> GIDPFTMAGAEWKSLEECLEKHLPLPDLQEVKRVLYGKELRKLDLPREAFEAASREDFELQGYAFEAAEEQLRRPRIVHVGLVQNRIPLPANAPVAEQVSALHRRIKAIVEVAAMCGVNIICFQEAWTMPFAFCTREKLPWTEFAESAEDGPTTRFCQKLAKNHDMVVVSPILERDSEHGDVLWNTAVVISNSGAVLGKTRKNHIPRVGD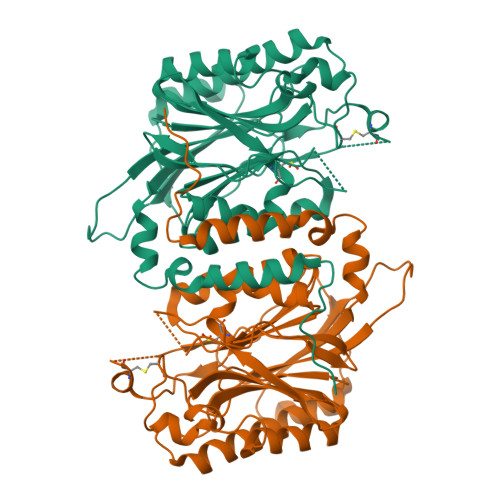FNESTYYMEGNLGHPVFQTQFGRIAVNICYGRHHPLNWLMYSINGAEIIFNPSATIGALSESLWPIEARNAAIANHCFTCAINRVGTEHFPNEFCSGDGKKAHQDFGYFYGSSYVAAPDSSRTPGLSRSRDGLLVAKLDLNLCQQVNDVWNFKMTGRYEMYARELAEAVKSNYSPTIVKE>[3x]SPNYDKWEMERTDITMKHKLGGGQYGEVYEGVWKKYSLTVAVKTLKEDTMEVEEFLKEAAVMKEIKHPNLVQLLGVCTREPPFYIITEFMTYGNLLDYLRECNRQEVNAVVLLYMATQISSAMEYLEKKNFIHRDLAARNCLVGENHLVKVADFGLSRLMTGDTYTAHAGAKFPIKWTAPESLAYNKFSIKSDVWAFGVLLWEIATYGMSPYPGIDLSQVYE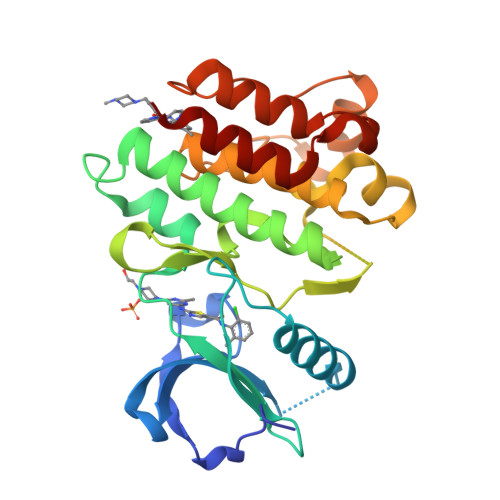LLEKDYRMERPEGCPEKVYELMRACWQWNPSDRPSFAEIHQAFETMFQE> GVGVSTGSYDNQTHYRFLGDGWVEITALATRLVHLNMPKSENYCRIRVHNTTDTSVKGNMAKDDAHEQIWTPWSLVDANAWGVWLQPSDWQYICNTMSQLNLVSLDQEIFNVVLKTVTEQDLGGQAIKIYNADLTACMMVAVDSNNILPYTPAANSMETLGFYPWKPTIASPYRYYFCVDRDLSVTYENQEGTVEHNVMGTPKGMNSQFFTIENTQQITLLRTGDEFATGTYYFDTNPVKLTHTWQTNRQLGQPPLLSTFPEADTDAGTLTAQGSRHGTTQMGVNWVSEAIRTRPAQVGFCQPHNDFEASRAGPFAAPKVPADITQGVDKEANGSVRYSYGKQHGENWASHGPAPERYTWDETSFGSGRDTKDGFIQSAPLVVPPPLNGILTNANPIGTKNDIHFSNVFNSYGPLTAFSHPSPVYPQGQIWDKELDLEHKPRLHITAPFVCKNNAPGQMLVRLGPNLTDQYDPNGATLSRIVTYGTFFWKGKLTMRAKLRANTTWNPVYQVSAEDNGNSYMSVTKWLPTATGNMQSVPLITRPVARNTY

We have been using the parvovirus minute virus of mice (MVM) as a model for studies on virus biomechanics. The virion 41 is built from a self-assembled T = 1 icosahedral capsid, 43 into which the single-stranded (ss) DNA viral genome is later packaged. The capsid is made of 60 protein subunits (VPs) with identical sequence and fold, except for their N-terminal segments (Nts). Pores (channels) at the capsid 5-fold symmetry (S5) axes are involved in DNA encapsidation, uncoating, and biologically relevant translocation of VP2 and VP1 Nts in the virion.

We have now determined the crystal structure at 3.8 Å resolution of the mutant N170A VP2-only capsid, and compared it with the crystal structure of the non-mutated VP2-only capsid (strain p). The N170A MVMp capsid crystallized in the rhombohedral space group R32. In the virion, the Nts have been externalized through the pores and, accordingly, electron density corresponding to the glycine tract is found inside the pores. For the N170A mutant capsid no density was observed within the pores, which indicates that the disordered VP2 Nts are not constitutively externalized. The structures of N170A and wt capsids are very similar but not identical. The root mean square deviation (RMSD) was 0.58 Å for equivalent Cα atoms in both structures (1.08 Å for all atoms in the 549 VP2 residues superimposed). In the ring of five N170/D171 residues located near the base of the β-cylinder that surrounds each capsid pore, the N170 amide group can form a hydrogen-bond with the carboxylic group of D171 of the neighboring VP2 subunit. This interprotein interaction cannot occur in the N170A capsid structure. In addition, removal of the amide groups of the five N170 residues generated five cavities around the pore walls. However, the free aperture of the pore at the tightest constriction formed by the ring of L172 residues immediately below the N170/D171 ring remained nearly unchanged, with a diameter of 7.9 Å in the N170A capsid compared to 8.2 Å in the wt capsid. The results reveal that the capsid-stiffening, cavity-creating N170A mutation neither modifies the diameter of the pore nor induces any dramatic conformational change around the pores; instead, it generates subtle rearrangements that propagate through the whole capsid, resulting in a more compact, less flexible structure.>MTVVSAFLVPGTPLPQLKPEVPSWGQLAAATERAGKALAASRPDVVLVYSTQWLAVLDQQWLTRPRSEGVHVDENWYEFGDLAYDIRADTALAEACVTSSPLHGVHARGVNYDGFPIDTGTITACTLMGIGTDAFPLVVGSNNLYHSGEITEKLAALAVDCAKDQNKRVAVVGVGGLSGSLFREEIDPREDRIANEEDDKWNRRVLKLIEAGDVSALREAMPVYAKEARVDMGFKHLHWILGALKGKFSGANVLGYGPSYGSGAAVIEFRL[2x];>MQGEIIAGFLAPHPPHLVYGENPPQNEPRSQGGWEVLRWAYERARERLDAMKPDVLLVHSPHWITSVGHHFLGVPELSGKSVDPIFPNVFRYDFSLNVDVELAEACAEEGRKAGLVTKMMRNPKFRVDYGTITTLHLIRPQWDIPVVGISANNSPYYLNTKEGMSEMDVLGKATREAIRKTGRKAVLLASNTLSHWHFHEEPTIPEDMSKEYPATMAGYQWDIRMIELMRQGKTSEVFKLLPQFIDEAFAEVKSGAFTWMHAAMQYPELAAELFGYGTVIGTGNAVMEWDLRKAGLSMLGAADQKQRSAAVA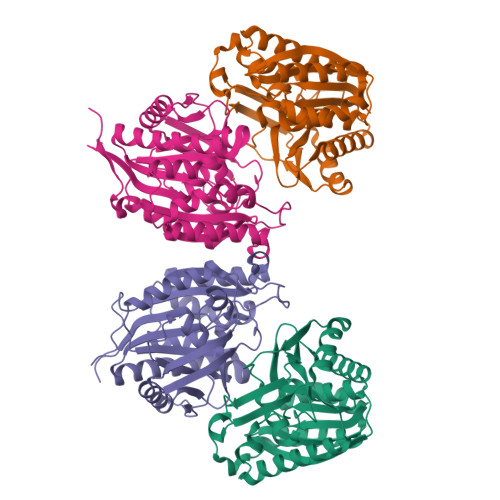[2x]Bacteria swim in viscous liquid environments by using the flagellum. The flagellum is composed of about 30 different proteins and can be roughly divided into three parts: the basal body, the hook, and the filament. The hook is a relatively short axial segment working as a universal joint connecting the basal body and the filament for smooth transmission of motor torque to the filament oriented off-axis of the motor. The model of FlgE consists of three domains, D0, D1, and D2, arranged from the inner core to the outer surface of the hook, just as previously modeled.

Here we report the native supercoiled hook structure at 3.6 Å resolution obtained by cryoEM single-particle image analysis of the Salmonella polyhook. Based on this cryoEM map, we built atomic models of FlgE for 26 subunits that cover more than two turns of the 1-start helix of its helical assembly. The supercoil was left-handed with a helical pitch of 129 nm and a diameter of 33 nm. Accordingly, the subunit conformation gradually changes along the circumference from one protofilament to the next due to the supercoiled nature of the native hook structure, although the conformations of subunits are nearly identical within each protofilament. So, although the conformations of the 26 subunits we built into the map were all similar to one another, we identified 11 distinct conformations among them, one for each protofilament. These 11 distinct conformations are all realized by slightly different arrangements of the three domains but the domain conformations are well preserved. When the two subunit conformations in the shortest and longest protofilaments are compared by superposing the D0 domains, domain D1 shifts up by 5 Å and tilts by 4°, and domain D2 tilts by 24° in addition, in order to achieve an overall subunit length extension of 14.7 Å. Thus, the compression and extension of each protofilament during the smoke ring-like rotation is achieved by changing relative domain orientations of FlgE while maintaining the conformation of each domain. The bottom of the C-terminal helix of the upper subunit axially overlaps with the top of the C-terminal helix of the lower subunit to allow their mutual sliding for protofilament compression and extension. The D2 domains form a six-stranded helical array on the surface of the hook by their tight interactions along the 6-start helical direction regardless of the protofilament length.

>SFSQAVSGLNAAATNLDVIGNNIANSATYGFKSGTASFADMFAGSKVGLGVKVAGITQDFTDGTTTNTGRGLDVAISQNGFFRLVDSNGSVFYSRNGQFKLDENRNLVNMQGMQLTGYPATGTPPTIQQGANPAPITIPNTLMAAKSTTTASMQINLNSTDPVPSKTPFSVSDADSYNKKGTVTVYDSQGNAHDMNVYFVKTKDNEWAVYTHDSSDPAATAPTTASTTLKFNENGILESGGTVNITTGTINGATAATFSLSFLNSMQQNTGANNIVATNQNGYKPGDLVSYQINNDGTVVGNYSNEQEQVLGQIVLANFANNEGLASQGDNVWAATQASGVALLGTAGSGNFGKLTNGALEASNVDLSKELVNMIVAQRNYQSNAQTIKTQDQILNTLVNLR[26x]>ETGCDDPPRFVSMKPQGTLKPSYSPGEQIVYECRLGFQPVTPGQVLALVCQDNNTWSSLQEGCKKRRCPTLADPTNGQVILVNGSTAFGSEVHYVCNNGYYLLGTNISYCEVSSGTGVNWSDNPPTCEKIHHHHHH[2x]

CD46, or membrane cofactor protein, is a type-one transmembrane protein from the complement regulatory protein family. When responding to complement activation, CD46 binds the complement activation fragments C3b and C4b, which have been deposited on the host cell. CD46 then facilitates the cleavage and inactivation of these complement activation fragments by acting as a cofactor for serine protease factor 1. Bovine CD46 acts as a cellular receptor for bovine viral diarrhoea virus (BVDV), a bovine pestivirus causing reproductive losses, as well as other clinical signs, such as diarrhoea and mucosal disease in persistently infected animals.

The STP region which is situated between the SCR and the transmembrane domain was not present in these protein constructs. The putative BVDV binding site was located in SCR1 and encompassed two peptides, E66-V69 and G82-L87. When mapped to the structure, these peptides were found on the C and D beta strands and D’D loop and formed a single binding site due to the antiparallel beta strand configuration. The area of interaction with BVDV was identified as two peptides on SCR1, as seen in both bovCD46 structures; these form a single interaction interface. Comparing this region with the same region in the human structure revealed a shift in the DD’ loop. An intriguing feature of these two crystal structures was the crystallographic dimer formation, which was identical in both protein constructs, despite them varying in size, unit cell, and space group. Our attempts to verify that this crystallographic dimer was physiological were not conclusive.> 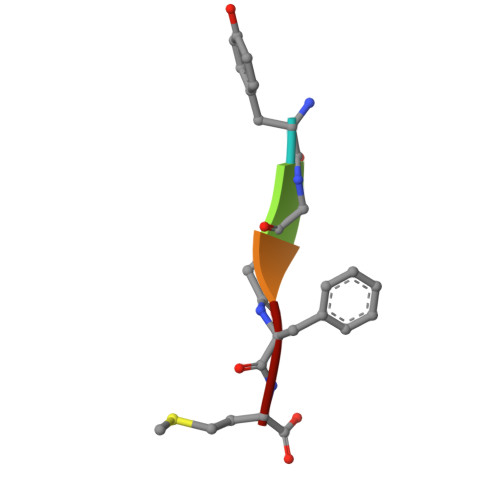YGGFM>CGC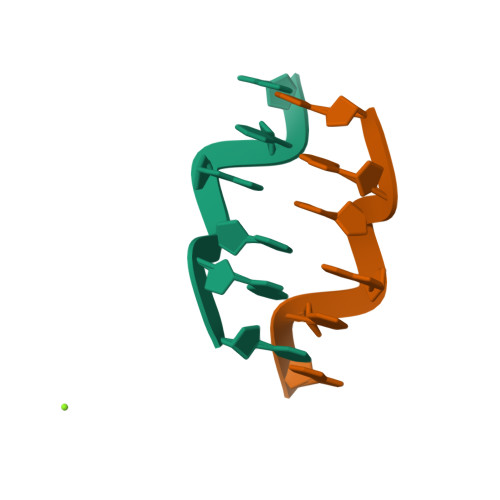GNG[2x]>[5x]GQDMVSPPPPIADEPLTVNTGIYLIECYSLDDKAETF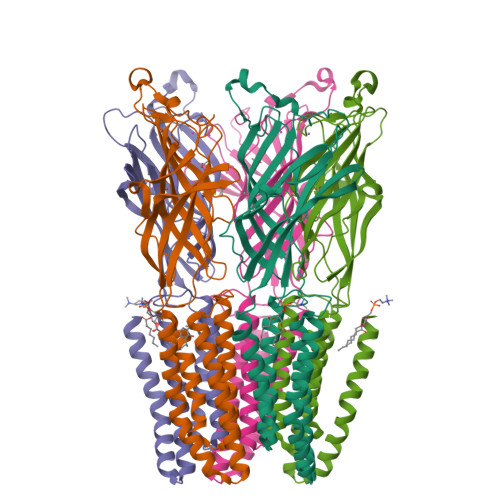KVNAFLSLSWKDRRLAFDPVRSGVRVKTYEPEAIWIPEIRFVNVENARDADVVDISVSPDGTVQYLERFSARVLSPLDFRRYPFDSQTLHIYLIVRSVDTRNIVLAVDLEKVGKNDDVFLTGWDIESFTAVVKPANFALEDRLESKLDYQLRISRQYFSYIPNIILPMLFILFISWTAFWSTSYEANVTLVVSTLIAHIAANILVETNLPKTPYMTYTGAIIFMIYLFYFVAVIEVTVQHYLKVESQPARAASITRASRIAFPVVFLLANIILAFLFFGF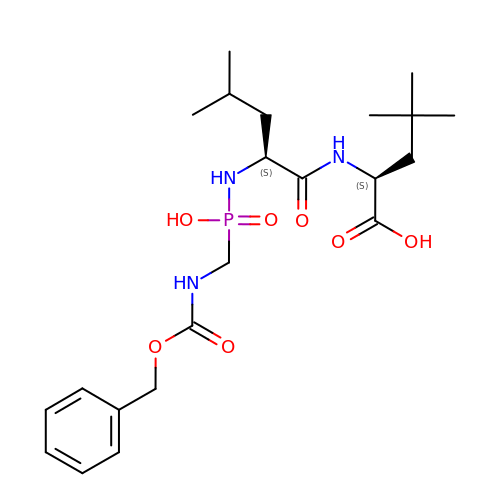N-[(S)-({[(benzyloxy)carbonyl]amino}methyl)(hydroxy)phosphoryl]-L-leucyl-4-methyl-L-leucine | C22 H36 N3 O7 P | DFAPONQEYRMEDO-ROUUACIJSA-N> MGESLDRCIDDINRAVDSMSTLYFKPPGIFHNAILQGASNKASIRKDITRLIKDCNHDEAYLLFKVNPEKQSVSRRDGKEGVFDYVIKRDTDMKRNRRLGRPGEKPIIHVPKEVYLNKDRLDLNNKRRRTATTSGGGLNGFIFDTDLIGSSVISNSSSGTFKALSAVFKDDPQIQRLLYALENGSVLMEEESNNQRRKTIFVEDFPTDLILKVMAEVTDLWPLTEFKQDYDQLYHNYEQLSSKLRFIKKEVLLQDDRLKTMSQYHPSSSHDV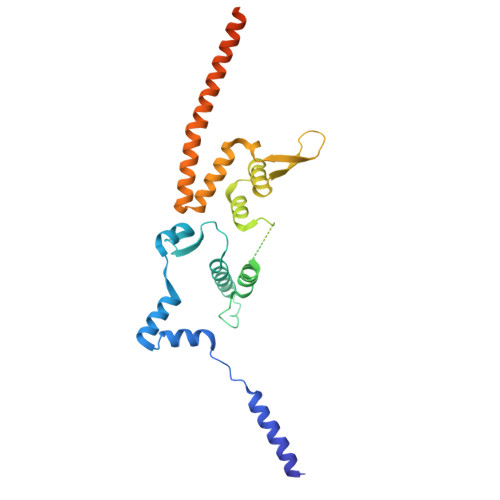AKIIRKEKDEIRRLEMEIANLQE>[3x]LESTESRSSFSQH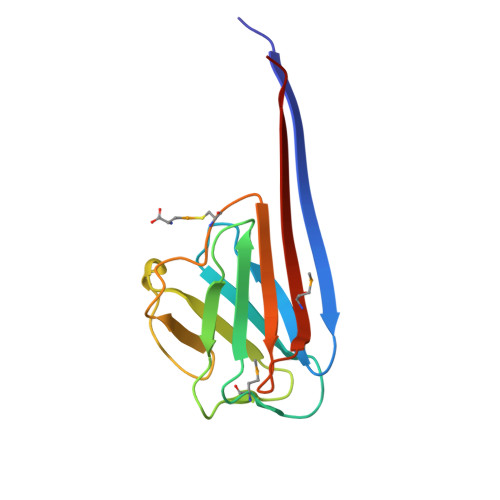ARTSGRVAVEEVDEEGKFVRLRNKSNEDQSMGNWQIKRQNGDDPLLTYRFPPKFTLKAGQVVTIWAAGAGATHSPPTDLVWKAQNTWGCGNSLRTALINSTGEEVAMRKLVRSVTVVED> XDYAEPMD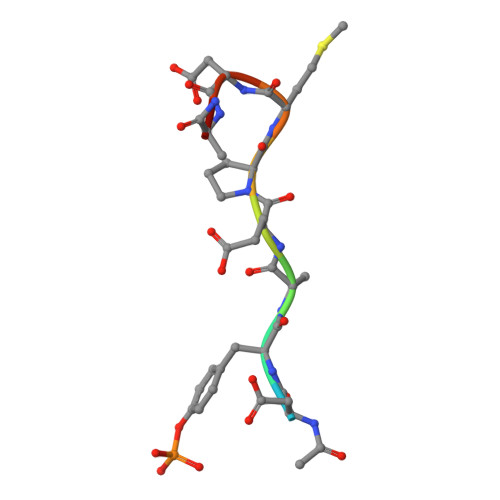AX>MEGTGVVAVYGNGAITEAKKSPFSVKVGLAQMLRGGVIMDVVNAEQARIAEEAGACAVMALERVPADIRAQGGVARMSDPQMIKEIKQAVTIPVMAKARIGHFVEAQILEAIGIDYIDESEVLTLADEDHHINKHNFRIPFVCGCRNLGEALRRIREGAAMIRTKGEAGTGNIIEAVRHVRSVNGDIRVLRNMDDDEVFTFAKKLAAPYDLVMQTKQLGRLPVVQFAAGGVATPADAALMMQLGCDGVFVGSGIFKSGDPARRARAIVQAVTHYSDPEMLVEVSCGLGEAMVGINLNDEKVERFANRS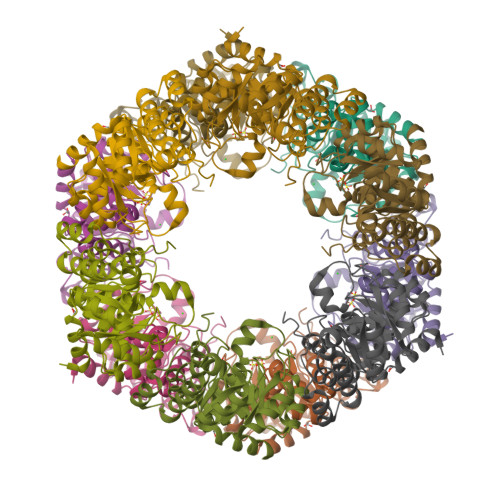EHHHHHH[4x]> SGLVPRGSHMIIKNYSYARQNLKALMTKVNDDSDMVTVTSTDDKNVVIMSESDYNSMMETLYLQQNPNNAEHL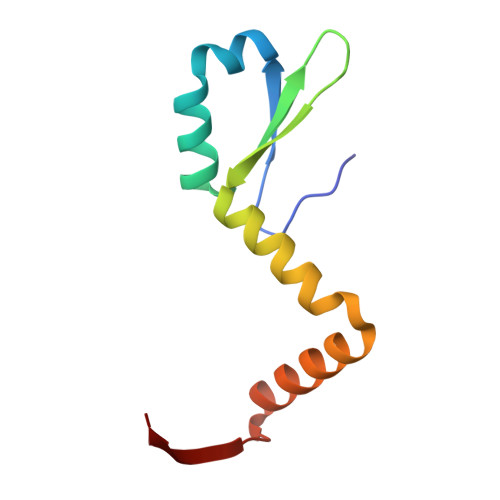AQSIADLERGKTITKDIDV> MSRLDKSKVINSALELLNEVGIEGLTTRKLAQKLGVEQPTLYWHVKNKRALLDALAIEMLDRHH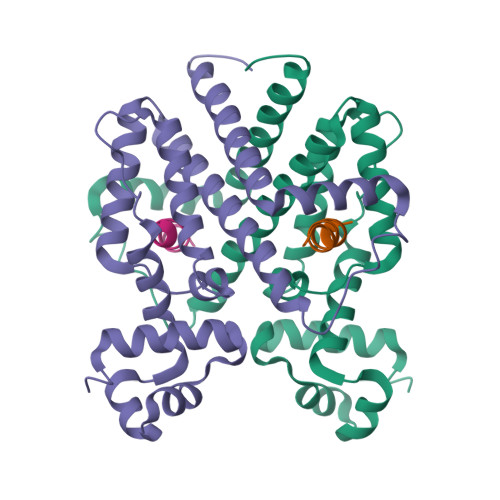THFSPLEGESWQDFLRNNAKSFRNALLSHRDGAKVHLGTRPTEKQYETLENQLAFLTQQGFSLENALYALSAVGHFTLGSVLEDQEHQVAKEERETPTTDSMPPLLRQAIELFDHQGAEPAFLHGLESLIRGFEVQLTALLQIV;> TGERGRWQVWGLAKRC Here, we identify CedA as an unconventional transcription factor specifically associated with the RNA polymerase (RNAP) σ70 holoenzyme. Structural and biochemical analysis of CedA bound to RNAP reveal that it bridges distant domains of β and σ70 subunits to stabilize an open-promoter complex. CedA does so without contacting DNA. Finally, we show that CedA modulates transcription of hundreds of bacterial genes, which explains its pleotropic effect on cell physiology and pathogenesis.

To gain further insight into the mechanism of CedA, we used cryo-EM to solve the structure of CedA bound to the RNAPσ70-open-promoter complex. Purified RNAPσ70 holoenzyme was first incubated with 85-bp DNA representing −60 to +25 positions relative to the transcription start site of the ssrA promoter, which has the strongest association with CedA, as determined by ChIP–seq. Purified CedA was added to the preformed RNAPσ70·ssrAp and the resulting complex was repurified by gel filtration and used for single-particle cryo-EM analysis. A structure of the whole complex was determined at the overall resolution of 2.76 Å, which let us to build the CedA model de novo. We identified CedA adopting a ladle-like shape and binding the RNAP at the tip of a β-pincer formed by a lineage-specific sequence insertion βi4, β-lobe and σ70. Instead, it binds βi4 via predominantly hydrophobic contacts. An N-terminal part of CedA, which was reported as unstructured, stretches along the DNA-facing side of β-lobe and the very N terminus (residues 5–10), bridging the gap between the β-lobe and σ70 region 1.2, effectively locking the melted DNA in the RNAP main channel. The N terminus of CedA forms several hydrogen bonds with σ70. The only side-chain-specific contact was found between CedA Asn9 and σ70 Arg385, whereas other contacts involve main-chain atoms. A close spatial proximity of the CedA N terminus to σ70 regions 1.1 and 2, which are bound to a nontemplate DNA strand, explains why an apparent DNA binding site of CedA was identified as a −10 σ70 promoter consensus sequence.

>[3x]MQGSVTEFLKPRLVDIEQVSSTHAKVTLEPLERGFGHTLGNALRRILLSSMPGCAVTEVEIDGVLHEYSTKEGVQEDILEILLNLKGLAVRVQGKDEVILTLNKSGIGPVTAADITHDGDVEIVKPQHVICHLTDENASISMRIKVQRGRGYVPASTRIHSEEDERPIGRLLVDACYSPVERIAYNVEAARVEQRTDLDKLVIEMETNGTIDPEEAIRRAATILAEQLEAFVDLRDVRQPEVKEEKPEFDPILLRPVDDLELTVRSANCLKAEAIHYIGDLVQRTEVELLKTPNLGKKSLTEIKDVLASRGLSLGMRLENWPPASIADE;> MVYSYTEKKRIRKDFGKRPQVLDVPYLLSIQLDSFQKFIEQDPEGQYGLEAAFRSVFPIQSYSGNSELQYVSYRLGEPVFDVQECQIRGVTYSAPLRVKLRLVIYEREAPEGTVKDIKEQEVYMGEIPLMTDNGTFVINGTERVIVSQLHRSPGVFFDSDKGKTHSSGKVLYNARIIPYRGSWLDFEFDPKDNLFVRIDRRRKLPATIILRALNYTTEQILDLFFEKVIFEIRDNKLQMELVPERLRGETASFDIEANGKVYVEKGRRITARHIRQLEKDDVKLIEVPVEYIAGKVVAKDYIDESTGELICAANMELSLDLLAKLSQSGHKRIETLFTNDLDHGPYISETLRVDPTNDRLSALVEIYRMMRPGEPPTREAAESLFENLFFSEDRYDLSAVGRMKFNRSLLREEIEGSGILSKDDIIDVMKKLIDIRNGKGEVDDIDHLGNRRIRSVGEMAENQFRVGLVRVERAVKERLSLGDLDTLMPQDMINAKPISAAVKEFFGSSQLSQFMDQNNPLSEITHKRRISALGPGGLTRERAGFEVRDVHPTHYGRVCPIETPEGPNIGLINSLSVYAQTNEYGFLETPYRKVTDGVVTDEIHYLSAIEEGNYVIAQANSNLDEEGHFVEDLVTCRSKGESSLFSRDQVDYMDVSTQQVVSVGASLIPFLEHDDANRALMGANMQRQAVPTLRADKPLVGTGMERAVAVDSGVTAVAKRGGVVQYVDASRIVIKVNEDEMYPGEAGIDIYNLTKYTRSNQNTCINQMPCVSLGEPVERGDVLADGPSTDLGELALGQNMRVAFMPWNGYNFEDSILVSERVVQEDRFTTIHIQELACVSRDTKLGPEEITADIPNVGEAALSKLDESGIVYIGAEVTGGDILVGKVTPKGETQLTPEEKLLRAIFGEKASDVKDSSLRVPNGVSGTVIDVQVFTRDGVEKDKRALEIEEMQLKQAKKDLSEELQILEAGLFSRIRAVLVAGGVEAEKLDKLPRDRWLELGLTDEEKQNQLEQLAEQYDELKHEFEKKLEAKRRKITQGDDLAPGVLKIVKVYLAVKRRIQPGDKMAGRHGNKGVISKINPIEDMPYDENGTPVDIVLNPLGVPSRMNIGQILETHLGMAAKGIGDKINAMLKQQQEVAKLREFIQRAYDLGADVRQKVDLSTFSDEEVMRLAENLRKGMPIATPVFDGAKEAEIKELLKLGDLPTSGQIRLYDGRTGEQFERPVTVGYMYMLKLNHLVDDKMHARSTGSYSLVTQQPLGGKAQFGGQRFGEMEVWALEAYGAAYTLQEMLTVKSDDVNGRTKMYKNIVDGNHQMEPGMPESFNVLLKEIRSLGINIELEDE;> MKDLLKFLKAQTKTEEFDAIKIALASPDMIRSWSFGEVKKPETINYRTFKPERDGLFCARIFGPVKDYECLCGKYKRLKHRGVICEKCGVEVTQTKVRRERMGHIELASPTAHIWFLKSLPSRIGLLLDMPLRDIERVLYFESYVVIEGGMTNLERQQILTEEQYLDALEEFGDEFDAKMGAEAIQALLKSMDLEQECEQLREELNETNSETKRKKLTKRIKLLEAFVQSGNKPEWMILTVLPVLPPDLRPLVPLDGGRFATSDLNDLYRRVINRNNRLKRLLDLAAPDIIVRNEKRMLQEAVDALLDNGRRGRAITGSNKRPLKSLADMIKGKQGRFRQNLLGKRVDYSGRSVITVGPYLRLHQCGLPKKMALELFKPFIYGKLELRGLATTIKAAKKMVEREEAVVWDILDEVIREHPVLLNRAPTLHRLGIQAFEPVLIEGKAIQLHPLVCAAYNADFDGDQMAVHVPLTLEAQLEARALMMSTNNILSPANGEPIIVPSQDVVLGLYYMTRDCVNAKGEGMVLTGPKEAERLYRSGLASLHARVKVRITEYEKDANGELVAKTSLKDTTVGRAILWMIVPKGLPYSIVNQALGKKAISKMLNTCYRILGLKPTVIFADQIMYTGFAYAARSGASVGIDDMVIPEKKHEIISEAEAEVAEIQEQFQSGLVTAGERYNKVIDIWAAANDRVSKAMMDNLQTETVINRDGQEEKQVSFNSIYMMADSGARGSAAQIRQLAGMRGLMAKPDGSIIETPITANFREGLNVLQYFISTHGARKGLADTALKTANSGYLTRRLVDVAQDLVVTEDDCGTHEGIMMTPVIEGGDVKEPLRDRVLGRVTAEDVLKPGTADILVPRNTLLHEQWCDLLEENSVDAVKVRSVVSCDTDFGVCAHCYGRDLARGHIINKGEAIGVIAAQSIGEPGTQLTMRTFHIGGAASRAAAESSIQVKNKGSIKLSNVKSVVNSSGKLVITSRNTELKLIDEFGRTKESYKVPYGAVLAKGDGEQVAGGETVANWDPHTMPVITEVSGFVRFTDMIDGQTITRQTDELTGLSSLVVLDSAERTAGGKDLRPALKIVDAQGNDVLIPGTDMPAQYFLPGKAIVQLEDGVQISSGDTLARIPQESGGTKDITGGLPRVADLFEARRPKEPAILAEISGIVSFGKETKGKRRLVITPVDGSDPYEEMIPKWRQLNVFEGERVERGDVISDGPEAPHDILRLRGVHAVTRYIVNEVQDVYRLQGVKINDKHIEVIVRQMLRKATIVNAGSSDFLEGEQVEYSRVKIANRELEANGKVGATYSRDLLGITKASLATESFISAASFQETTRVLTEAAVAGKRDELRGLKENVIVGRLIPAGTGYAYHQDRMRRRAAGEAPAAPQVTAEDASASLAELLNAGLGGSDNE;> MARVTVQDAVEKIGNRFDLVLVAARRARQMQVGGKDPLVPEENDKTTVIALREIEEGLINNQILDVRERQEQQEQEAAELQAVTAIAEGRR;> MEQNPQSQLKLLVTRGKEQGYLTYAEVNDHLPEDIVDSDQIEDIIQMINDMGIQVMEEAPDADDLMLAENTADEDAAEAAAQVLSSVESEIGRTTDPVRMYMREMGTVELLTREGEIDIAKRIEDGINQVQCSVAEYPEAITYLLEQYDRVEAEEARLSDLITGFVDPNAEEDLAPTATHVGSELSQEDLDDDEDEDEEDGDDDSADDDNSIDPELAREKFAELRAQYVVTRDTIKHATAQEEILKLSEVFKQFRLVPKQFDYLVNSMRVMMDRVRTQERLIMKLCVEQCKMPKKNFITLFTGNETSDTWFNAAIAMNKPWSEKLHDVSEEVHRALQKLQQIEEETGLTIEQVKDINRRMSIGEAKARRAKKEMVEANLRLVISIAKKYTNRGLQFLDLIQEGNIGLMKAVDKFEYRRGYKFSTYATWWIRQAITRSIADQARTIRIPVHMIETINKLNRISRQMLQEMGREPTPEELAERMLMPEDKIRKVLKIAKEPISMETPIGDDEDSHLGDFIEDTTLELPLDSATTESLRAATHDVLAGLTAREAKVLRMRFGIDMNTDYTLEEVGKQFDVTRERIRQIEAKALRKLRHPSRSEVLRSFLDD;> MKKPLRQQNRQIISYVPRTEPAPPEHAIKMDSFRDVWMLRGKYVAFVLMGESFLRSPAFTVPESAQRWANQIRQEGEVTE> MNFNVGVDFPSFIAWDGEESFPVKVDGFNQFGFTFKTIAALTAATTFNIFYHEPSDADPCVPGPAIRVPEVPFCDTVLLSEDGLAAVTLPETVTPDS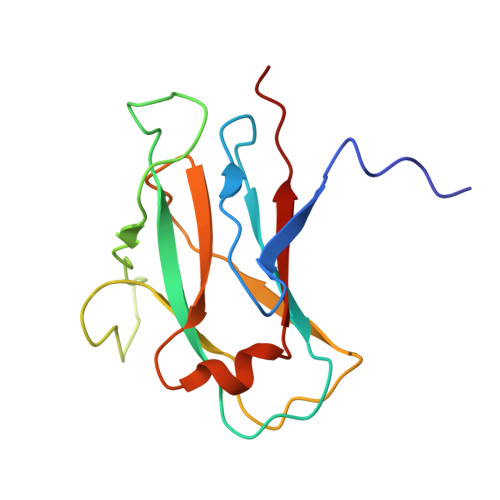FCAGTVPCMNGQWISIAPATGSETNAANVQITVTMKGATR> MNPSQTQKGKIQIQVSRGSIDLLVRTMYEDINNIKLKNERFQKKKRAEDERRRRERYAEIQQEAIASGKKNAALEMKWAELKELDECEELNREMQDQQQTFQQIIEGKENLRKEFEEELKRKDDEYVKMLKEQSNDIKDMISKMRSQFYKIRDANMQELEDIERHFEQERSNLLNEFKAKIQATFKKHLDLEEQYVKEHAKTEEEQTKNIEDLRIKGAKHYAELKITMETEIQDLEKCFEDMKALYQLITEKLDYSLKVLQEKFHENNSMCDELKRKENNFKNRLKQLTKDYKQYDKKFKLENKNLTQEYKRIIRQFKELQKKFKHFEKADLDKYSEIQKMNEAEVKELKDKIIKCNITIHIQQLGMQWIPPQSEEEILAQQKLQLEQGGKAEEEEEREFEFCISEIKIGEICNIILEEADFLIDDKLREELEGSAEPEQIFQRLDCIKKCLYIDSEDEMNLFFRELITKCRVKSAEEIEEEARKQLLLLGLIKEAEENENPEGEEVQQQEGAQQKKKEEGNKKDDPKGKEGAKDSKENANPQGQNKSNQDERKKKKDGQDDHAGQGQGQYDSNQGGMGENQEEGENAEGQENLEGEIEKEIDLENTQINLNEVVKFLQNWQANKDKRKEKLEKESSKKAVKQETEREKKERIAREGKKYWEKLTQVLPERTFRIWNVNFFKFSFEKQILLNQINKLRFWTDLCPNIMNFFWTDKNQSKKPVNCITKMKNQRIFQINTYKLIMNLLSALQDSLIQIKDKDDFIQTKISTNLFTFHNFQILLQIFIVNQSFLFIRLCQSYSKKIILLIKNINQKLFNLSNFKNQFSF;> MALLGKTLKGRSTRPGGIPQKRNIKWRQLAKNQEEFDQLKQLAKMKREGLKARIKDEQKVVTFNKKKLITYWRKIMRIAKTEQLKNEIDIYSQNNQRELDSKEAFIQMLDKNLDEAEDQFQIALRNHLIHIENLMQLQEARMRGLAEEFNRDVNILETEFDLEREEMVKTHKTQLKELEDMIETVKEEDKKKTEEAQNEFSQFKEETKNKNLEETNVMKIILETKQTKYYTELEQMNSKFQSDTSNKVKDHQFYHAHNKNRKQEIDRYLRTISSKKAKIDLMKLKILQHCKEFNARNSALKKEKENISRNYHELKLKMQKFREEESRRLKELSNNSRNAVLKLREYCALGEKILKTAELCRRLETEKEKVLPFYESSVDEDQIPEQLKNEFEHLKKEDAEEYAYLNNFYKRYNKVLLDKLAIEKQKENLQRDNQLLKSLLKQYLDGISLNDDVLKNENNPLLVVNHKFNLGKMPVEKIENKTVIEGVFEVRNTSHQLQGQRAPPFQ;> MSNYISNYVQSTIVTKTVQNKDKKTGKNSVDPRVINEQLILDAVKQFNQENNKITTENIILQQLRQLQLSFKNILKIQHLQGLERLEKLQLDNNIIEKIENIDHLVNLKWLDLSFNCIKKIEGLDKLKELTDLSLFNNYIEKIEGLHNNTKLNVFSIGNNRLKSYEEITLYFGYKPRGEEGTNDRPEFKRLQVLNVSGNPFTKDKENEYKNHIICAIPNLKYLDYVFIDEGDRQLIRQDEQISNSYNFTTTDYYQQMQAQEQKEEMDRQTLKKKKDARMDILDNLKDEYLKIEDLQRVKIIKPNQINEEIEKYCGKINDHVVEMQAAVIQKHQLILQEMSKTEVSYKEQEALHEKETLQILKEFEHEKKVEFRNWEKEAANGDAKKEESRLKTLLQKTTSLKNKLMDIEIQLVEELEAIFTDYDTKKKETAWKDIEEIIVLGQKKIEEENVKFYSNLNVIKNKEEANYNSTQQQQLEEENNEEDDEKASLLENKEQLAQMIGNIKETLIDSHTKIILSAQMELQKDLAEYAKQQKNKMYERNRKNISQIIAQIDAYQTEINEKLKQGDDESDHEN;> MSKAAKAKKNVPVVSKLEADARKAAEGVNDNESEEFKKAMRKEARALVEQFNEEKKLLAFYQQERQKINYNWIIAKKELEDKKSELINKEREIQDLQENHFMTLNVYKQKIKHLLFQNQDQQSELKKDVEVTLKQLEDQHRIKSRELKTDVRSLKVTKKEQEISQQDYLFALKSEHDKQMTLMRQDYERQVNDIKRKYDLKMQNLTKEMEEARAAMIKQLEDNKNQKIAEIIKEHTQKYNDIKNYYSEITATNLDYRKTLKNEIKELQTKDEEYKKTLQQTEKGYKELNEPLQALGIEIIQLKKQDEEQEAIIKEKEELKQKIDNQERLFRKLEYEYEVKLQQFQYLERERNALYAKFNQTVFEIHQKSGLENLILEKKVTNLREDLEIKDLQIHQVLTAANIDPNSVGSINKSLEEVESLKNELISELQAQLKQIRKAHSHMVKAYEGKLSEFVIPVEELGFDPLVPTNTD;> MPPKKAKGKKKKEEEPDDEYKSMTGADLTQTLEKLKERVNEMRTNRNYIQMDRDMVENFYHNTLKEISEVKTKISNKETEAEEKESKHRIDVKVFLQKVKHLEYEQEKSNLNIEDDGKKAKEKEDAYFEDITKNMKQLKTQLKSEYLEKEKANIQQVQEEKKDHQSLLKIQQKKFDELINNLIIKYEERLAKLKEDLELKLKVEIHELEERKNLHINELMNNHEKAFAELKKYYNDITAENLNLIKAHKEKIAQIYANIQLNTKNVADNQAKNEQLKEPLAKHREIRNKLKEDLKQFAKHKMSLQNLKSKAITLKDKITKLERDGKDLDEKYEKVVREKQELEKKFEDITQEVKKNADLNNNVLSNRLQILLKEYNNKEEELRTIIDNAGLDHNLHEQLKQRVQQSIEAKNTLIKNLKYSIHHATKAYNDAIRVYEAKLVEFGIPIEELGFQPLETITSSMPAGLVSS;> MLAKKLALARSQGKPDPFKKDEFPLLQHIAVEVVSQNYILYPDLKGVPENVRDTIISKITTDLDILTMAPNIDQESFWQRACKNRWEKSQKSINIEEHGRSWKVAYLERYMEEFLTNIQNADDPNKKQILQAELKAAASWIHTLNLQNINQNIDIDFICKYLPLLTSLTLTYGTKYSGMDYNKQSVGMKLSEAANLGEAIKNCYSLLSLNISANMIDDDLLRFIMAGVNMNISLIELNLSHNKIEDQGARRIAKFLMRNEILLYLNLGNNLIGYEGSRYLAQALKVNKNLQSLNLKLNNLGDKAGKKLFQDLMLNKTLLELDVSGNQFEFETALKLSDYVADSMCGLKVLNIANNDFNDSCYENLKTGFTKNYSLAKLDLRGNKFSKTQEEKEQELKDPFRMFNLSQTEKELTQIIIRHDLTAQKIQFFSESDLDKIKQLKELQGAKQEPEKVIQQDQNKE;> MGDKKGKKKGGGEEDESTLQLSRQYKKKCELNGINPSKLFKEKLDFAVEEDENIEKIHLWEELGPVGVRSIMDSLTEIPYLHTKSIRLWKVKAQDEGTRTICNYMEKSKTIEYLDLMDNQVGSLGCEFLGRVLHPQIEIPLLKLKLDHNEFGTEGLMQLAAGLCMNSVLEKLSLNYCAITAEGSKYIQQILSFVNTNLKKLKMKGNLLKNEGVHQLFRAFKVNKTLEKVDLSDNQFDTTLGDDQDPEANPNFFETNKDAIEHNKQIIENICEVLKAADTLLYYDFRFNNISKTDAKAIIDCLEANKNIYYMELSEHIPKDLIERKKGLMKKRKPKKKKKKKAKKK;> MDHNEGGYSHHQIEGQEGQQQQAPVGGGGEDIFQVLENITQVQNEKLKRCQEFKEQENIPRQYIENSPKEELVLEHVIQFKRQFQYQLYYEDKRDLFLYPKNECDVYKFICTTIRPTKLGFLELYDYQQCSKYLSEFVQYEELDPPNEFPLVIPSPTNVAVWQKGDCFDMSILLCSLLIGVGYDAYCVYGKAPREITTRNESLMECLFLEKGKYIEENDKKPKQTLEQNENALLKKPIAHSKWDQTQETKAREAEEEKRRIALTINDDEPDELLEDPYQGQRVHCWVLLRSGKRDVQQNIFIEPSTGRMYSPSTCPYECVDAVFNNLNFWINMKPECEVKNLNFEEMDSSLNWEYVMLDTLLFNKGNGNDEEGNENIDDPLNKQAQRDPEQEQLQDIAQLLDMPPPWPPKIYIDKEKFLMGTPLGEGTVYYNKVKVDNYAPYSQPDGLVQKITIFQDYKRLKVKEYRYFYKHRSDKLSIRRRYPFEFKTIEEYEPQKYENKTIPQALQQWRQVIQIDRHLRIIKYYHNRNHDGLIERVEQIGEKTMMFYQNRDDRVIYRSIRFDNKRAPSSQNNDKVFQDNHVGDVQITKMTQKFEKNPHYPANEQIQKMVIDLIKDKVIVYYHMNDGEITPIVKIYPRDSMHGFAKLNEPGGDNKIDDPLVQLENTKMVNLEKDCLNQLKQQEKIARDDEKTIREGEIRLEKTLYDKARDRFKESSKKNDDDLAKDAAASDYLYPYLEKRKLLGVSEINAQVAMEIKNEVMQKLKERLLSRAEIIQRRLEEQRQVLEQKEAQVAKRQEIDPKQEEEIRDINFKIDILEQRALRFESMALQKYEEMDNRLNKDARLAALHRK;>MYDPNTSQTEKQKQEEFLKLKIQEAFNLFVKDKKGIVDKREIPYIMRYLGQFPSEAQVRDAILPEIEEDEPSEFIKYSKFEPYMLKVLKEREYEPDDPEALLAAFKLLDQEGKGYIEIDMMKTFLEKQGIEFREQETKSFIEFATNKDPNATVIYYEDYISRLQAFTDKHIESVMKGYNNFQVKK[2x];> MNQIDAHKLTIILRDATERLTFLDTINRQDDLSSELAGYEISKLLKKQKNLENQYADLVQLRTSLTGIQNKKNLIETQTKIVDVAQNLKESTKKLCRLFKENPDLESDALKVKKDRIQFMAVIEQLIQMVQNNSLTKFQSMTTLELEDQDRLRKLIFREKELYQEIKKLQFDRNQENKEYDNEQKDTNLKIQNLKERLLYKKARAQLKNQYKEKEARAEEGTQQRMYEFEQKQLKEKINNLKQKTDTENMVHEQLRNFLIEKEDQIKQKSDEWAKKVETCREQLQEEIDRLTVEKEKKQEELRELRERDQKEQEEKDRRERQELEEADRKQQEELDQIRLDNAIKLIQIEYQEWKDAGGGKKKRKKGKKKKK;> MQNLSKMQSRLHPRPEGEGGGGGGRTKEKGKSLQETHKEMLKNIESTNIGKPTIVEAQRILKIIDNLSTNLTIFIYLDSELISKFLDVAKHSKLSKDLVSKLSQRCLDLLKSQAEIEAKFKPYASLLDQSNKEAEDVEEEKMIDAERLRMQLENNFKDLVRHLRNSPEDFEIIKSMKTNVNPDLNDLVHCIHCQKVIMLKKLSTASEEDENHKAQLRDLEEKIEELEKKKNKIQEDLTKLKEHRQKFSKEKKEELEKLKNEIAEVKAEKEKKASQLKNELDNRLKQLERDHLAKKDKLDKELQKLEDDFAKLKQDHANDETKLKTNKRQQQNSLADNIESYDALMKDQHQKKQEIEEELAKIIEEVDTLKQLFKEIDEEKQRERELEEEFRLKKEQWEIQERRKKEAARCILHFLMARKEKSKKKKKKKGKKKK;> MSNMMYNMKWQEAINDLMEQVTLEYLPLEQNEQQLGMKYKRDSSEWFHFWATLYIKYIDIYKKLEDCYDQLVHPQKRVLLKEMLENVIVRLCETKSQVVKYNTQYDATYKSDYPNLDELVMDLKLTPDCLDIPIPRYFREEDKKRLDERNQILDALLLEYTDTKEPQEEQYEDQNTLQADMDTAIRIIQRYERGRQGIERANLAKILKKEEEKKLERQKKLAEGTEIGEETEKDDAALVIKKYWRGYKSRKLVQDIREEELLFLGMKKVVEDPTLPESQYKQAQNKRQKMKYIQEEHEQEFNDEIENLKRLVKGNEGPDILDKMRAERREWIMRELEKNEFKEAPQDPSEFYNQQVMDPEQQAAEAAKAAEEAKKKGAAKKDDKKKKGKPSELDEFLENNKPTGPSPIVLKLQEQIEKHSGEWSKRDETNNFEQKHETELAKMLIKPVVEEQIKQQVDEMIAEELDIVRLRYDIKKKKQKKPPRPRNKGKNKKKFPGDSSNKGRDPKDILAGLVEKRVAKKLIPASLMDLKGEQNVLGKIQEIQADENLKKTEALTDAKLKKAQLEEPSTKMPDPSIAQIRQIIAEYIAFPLGSKYAKEKLDKMNYFFFMGPRGSGKTLAVRALAHECNAIVLDISPSNIDGQYTDKKQIDGMINSAFKVAKEFQPAIIYCEDFEYIFGQAKKKKSQVNPLFAKMKKPLMDFKKGKFFEPEDRVVFIGSTNRPWDCSQKEIKSFFDKKIYFPFPNYGTRMLLFKTFLEQKKVPLPDNFPINTIAHITEGWSAGSFKMAIDRVFTERRLQKINEEQIKLSEFIGPLSNVPFTSKEEFKEFKKFNQVVTGLQANYEAKKAPADDQKGDKNKKKK;> MATTTNILHDVVRDQSMVNYVSNRDRPLYFKRPLVPQMTDIPLHISRPPVDQQVDYQTMQMQQNATIVEAPTKDAFVQTDYRESETQTDPYTPKCFVRDGDHPEVMELKDYKYGKGLPASIEELEQIELNREKVWFENSLPPISDEASFNLRRKLMEEQELREWSKKENEIKKFQNEKLYLLQQALIEREKEVEDKSQERIEEIRQQKTEHKNRQIAKIQRKKIKIDRKMTKSRKMQGKETLKRDIIEDYANFASRVYAGITHEGLSLDKIANKYEVQPLALGNYEMLQALHEGIRPREFETRVNLKKEIKEIEKNYTRLENYHRGELKKAQDEINGVHEQSKAQQKQEGNNFSYRNFENKIRPATPTWKYDTDFNISPSLITEIQEYRGPNGVQLMQAADKREEAVLLLQRLLRGRTTQNIMYEGKKKRTALIEELLTVAQIENLEEDKAEEVLMQQHEEKVKNAVLESIQGEVIAETMDELSKELLRIKQERKIQQMVEIAEKDRRIREIEEAGKRQAEEILRDREDVLHNQLIRVHQGTVDTYLDWLMSNALEQSSARQATIMTNLRKAKFNLPLEDFERKYNNNQTLIKDLVHSFLIPNVQRSKLKKQIQLEEKRFSEAAKRSLQQTITRASNKHANVQN;>MDQGEFIQDDNDQDYDQQEGDDENNDYMEDPQQDNNYNQNGDNLDDQGQDDDGGQNNLQQPSVPPEDDEDDDDDFPEYANEQNKRLNEIIKKKRKLIKDISAKIEEKSDRTKVLQEHLKNVEQELLHTQALIDAKNKEIETEDHMKQIAERQSGRIQSELKILEKRSIEQQEKLNDVQNQIFRGNEKMDQYKLEMNWNQEELEQWALAARQKEEDNLTLEKYKRADEVKIKELNLAIEKLTAEVGRKQNELEKEITETQAAQIELDKTAEEFKRQHEERHKLFLQWQEVTEIISKRDLAIREEGENFARIKIEIKSNKDALEERKRILKEAKEENKRIQMANELMERQNIQQISDNKHIEEQLAEKKADVEILKNQVSAFASDLSSKKNRIAILSQELLAKKQRLNAAQKKYQAHQVKLKNEEIMAKQYENDRSYAEEKYRKNEKEKKELEKEIRTQKENLFKHTQELFKHREREANLYGEIQGNMAACRNLQSHITKLNQEFQRQQELLYNAEYQIQLMERRVARAKGERTLEEKKDLENEIMNAERELGGVTGQNKELIESLKNLDDEIRTVKKKLAYVEEENTKYSSLIEELILENDMTYQDLNKIIKQKEEVLVQHDTMKLEIKKINESLNGATEKVFNLENQIYQLEMSMQEREKEIEVHKDVLMTEHKAAEEERHKIAVELAERKNKVKNLKIKYESLVQKNKASNGEVESVHEHSQAYYVIKAAQEREELQRKGDELNAKILKNEKELKALDNTLNHLKNRNSNYRDKFLNKGVTTQHREEAEGLEEQCRAASQNLFKKRDELQKLQKEQEEDTRRYTEIKNKLERLYEQHQSLDQEISKYQKDIDQQGDKLQRAQNSLQRNYQLAVNKNQNFINPKNPHMIQVKLDNQNNLYKTLLQGLYSLQQDIPELSSVVDEILKEQRIQNNKAPSSIDINSKRSSQSGRSQRSQRSNISNQ[2x];>MSNQQGPEDNNLEDDMAYLPADHPLLAKLQIDLTKQLTDEHERVDQKLIEIDANLKKLEKTKEDIGVRLYSVQQQLAENQMNFEQAHENYNWVQKLRIEAEQKLKTESEVYDAKKKELEELRKKYLKAQDELSKLTRTLYQINEFNQQMKGQIINTKTNTYRAEENVVNLEAQKKKQDLLIDTMNEEIKRQTEQKTILTAQLISQKEETEQAKQILKEAHLEMQKIIASKKNLLERWQKSLMTMQRMDNALQAIKEALKGQQELNLQIGTELNGVNAEIRKETEIQESLEGKNKKFDYEKDYLQKKYNELQEEKSKLEAQINLLTQSLRQTETEAGRAEIDKRNIEDQMNLIETNIMKLHTETKKLWEDLVHQKSEHTTIEKTATNLNKQANQISIEIEDKSVELENLLNEIARVKIDQLNTLSQIEVLENKRREVIKEREEKEITVATYEVQIRQGHDLNEKKQHEVGRLNREHDKLSSVQSDMSRGPLEAKRNNLIRKTQELGKENDLMQREWIKKQTLLVTQNNRLNKIEEDVSQLKTKQTILEQKKLRLNNNYRIYEKDIREIQNALKNLRNEMNKLNDAIYRNKEKQQKLDNENFNIKSEFVEKLKELEKESVKLEVEIDRLKEEKADLLAEIVESERQILLWERKIQLEKEMQDALDPTVGQTEIQELKREIHRMELRLDDLRKKQEAIIAEMERAVYKRETIQLKYMNKDKTFSNSNSMSQKSSSISAASDNSAQITKKIAQLKTTLNQTTRNAEQMEKAIKNKKIELDDLNAQIEGNNDNLQKLESDCYNKNIELTKHKLERSTNILSISCMQNKAKKLEDLVAGKARLSVPEATLMTKYEELRDKNQEIKEALQKLCDDAPQYVEVLNYLIDLNVGDDDEDQEQ[2x];> MASEDGEMPSQFEGIDPEQLTESQMQQYMMEMQRQGLLDSNMEGGQYEEGYEEGQEGEGYGEEYGDQDYDGNQNEYDSQQDSQQQGHDQVNEMHQDRYDRRVNSEISGNYEADDETLRKIRRDLLDNINLERRHRDLQPVYIDLTTNNISQYYSEYLVNNEHNQDFYENAKVRYNNLGECELCHITAKFEPDADITKEYIYDYFMEIGYLFLESEEEKRIILNPANNHIGIGVFFDEIQIVVVLILSEKVLCIQKISQPEQNKIEIRGKMLDENFGIYAIRIMNVDDQKKDIKGVGPEFIEYTRSTQEWMASFELELYNQDRMAIEYYTRVSPDSIPYKKKQSKNEKLTYKHLQLRLRTPFQIYPDPKYAAEDEKERIRKEQEILAHEEQERKEREENDAKRLKQSRKDYGDGQYDDDEHGQDDFNSQSDISDKDKHHDSMHAEQEQNQQAAQQQQDTISNKEIRQELEMAITEAQRQHDEFMLQNHKLQEEIKLLKNKNDGFVDRSNETAMNEHKYLNTLAHVHQIRLDLKQTQTRYNQMSQELQKKLEQKQKKCNEIKYAFLELKREVAKKAANSRTDKPIPEQQINEWEKAELQKSKELQELRLQILRLRNAYVKNQKILKKKEELAEGLHLIDFEQLKIENQTLNEKIEERNEELHKLKKKNTTTIQILTHTREKLGFVQGENGELNSQNVRKDQELDDMRKQLTQQKKTKDKLRSVNLTLKQQTGIVNSEELGQDYRDLRTRVSKLEEEKKRLEQKLRSMHEAIKTANQISTQNMQSQNNSLKKPYQPY;>MDNTGKLEKQLVTLNDGLPKKPAKEIIEELKHHLYQDFQKFFSEEKKQQYQNNFALFDRDNDKYINLSELKELLTSVNITFPDDELEELYNEFCLTSPEADGINEDAVFIIVSKKIRDNDKDEQLTQAFKLVEKAVNDELAKTPNETKEQEGYIRVEQFKELLMTLGNRWSEEQANEFLKDINPKSDERINYLDVVKKLMKR[2x];>[2x]MSKKSGKGKGKNDGDELGAEKEQVLRTKVESLIQRLGHEQERADRAKAAENELRARLFDLDKDFKNEKDRLFSITSDMTRQYKQMQDELLNQVNDLNKTVIEKDEEIKKKDQQIQDMTKDYEYKLKKKDDEIQDLKRKIEEMSAEFAKMLKDTLDKMQERIEMVQWDSDTDPQMMKRLKDMTGLSNN;> MNQDKHPEITDEEQELITVEELSQKLELLYKDMEQIRRENLLFEAYLARNRKEIAKEDEVSEDKKGKGKKKDKNVDKKSLLLTNEEKFEIAQQEQDALKKQIDDGRIKSDQILETLRAILEETDMAITEIRKDAFDFQREILVGGENSRTGKIEAEKIIKFFEEKERQKDALIAKYSSKRTNLERQILKTNNQIQKKEEMGDDLKFIDFYQLQIENKKYVKEIDDKNKKLLALKISTNRISQTLKDEKQNLKQELDKGKEYASQMSERKKKISKIDAQIKSVKKVTSKLEKDRKIYDKQKEIFVQDNQDDVPQIMKYVQYKSKEQQLLYAIQNLERKIEIAELAYKKANRILQSSQQFQQK;> MAGLAQHIQLKYIFGMNNEIRNSLQFHDEDRIIYPAGYNVVLHDLNDKSQHYYQGTNEYRGISCLALSPLKRYLALGVKGQRDPAIIIFDTFTQKRRKNLGLNLGNLDRYNIKQWVSIAFPSQNQETKYIFSLSGAGGDVVLCWWWHEKGKCLGSIDLGAQNDIYEISFNHSDANSICVTGNNFFGIYAKIEGTYVREDNQQKQKPSVQNGENSSAAQLPQPTLNIQVSAGNNNQNPQPEIKLENGNLISNLPADIVEKNFVAHLWMQCESYLVVFVESGEIILCDSRGNFLQIMEQSPRYFIVSRSGMIKIVAAVAYSKGFYVACSESIVLQYHYTQDNDKNPFTCVNQFKLKQFVELKEIEIKSICMNKAEDKLLIGLDNNQIYEIKIKPYHPETVNNDSSEDREVTLINHLNHTGPINSMDICKRKPIIATCSTDKTIKIWDYEKKQIKISWAFNEEAFCLSLHPQGFCVAVGFLDKLRLMNLCIHNSQNTTKNKAYKEISPFKGCKEIKFSNGGQYFAAVNSTSSNHVIQVFKFFTGENPSQLVFKGHTGRVKCIAWSSDDSFLLSCGLDGMILAWKLDQDFQHQQTIVPRIVDIHNKGVNFSGLTLTVDNKTIVAVGNDRHIHQAVINEQQPVDKTDKKLLDINLSCLAFPSSNKLLFAGIQDDARSSGAIRCFIYPLTHGKFTDYQAHDERGVEKMKITNDDRYIITAGKDGCIMVFEIKDKDARGMKLKDGYAKYSEEELITRSDLDDLKSTRDGLIVQINEFSNQNAMIGLNSRDDRIRQLETQIENNSQKRKQMFEQLLKSKTMEEQKLIQEINEIKEQFEQEIQVMDTKYQKEVMSLVEEYENQKRLHEIENNKNNKKKTKLLQEHSQKLQIIDDQYQKLLEEQITQKERVEKQINHLQKEQQEVLMQISEEKETEIKNLNQKNSKDEQAITDQGLKAKSDISITKKKIMQQQQEAQDLKEQKQEYERQKEKLKIQNQELRDKIDGQKKIILERDRTIGEKEKIIYNLKKKAQDLEKFKFVLDHKIKELKRDIVPREDEITKMKQETNNMDQYLKELNAYNNYLGTVVDELYTTQETMKEDIKQQRQQISVQQVKISRFKDDVYSLAQHILDYDKLVDETERLFMKHVNDKEVKRQSVEGDIMMEYRSQKKNLEKLVNMFKKSLQKDNQIHKDDKIRIMKDNVDLIREINTLRKSIKDITKGQQSNIPDQKGQTQHMPLQTPQLSRKSISQPVLPPISKSAMFEGVTQQNEIQKSHTQINPELVEEKQKVLNSLQTDILELQKVYEALNYEKHNLTQA;> MSSDVKDSSHLEKQNSQEYSNSKQNGEIDIMEMLPQKKMYIIEKQFDQSGKGLKIDEFVRVMLTHLDFDKSDVQKEDQITLALIDLFKEIDVNGDGTMEWEEFSDHIISLGLLRNDRSFKNVIKNYFPSEHIKDNQKHETPIEKIVYFDKLKYLVVLEKDSTRFKVYNANTAELYYEVNAHKCAVLDAEYIPDQNLIATSSNDLTINFWDSSFFIPKQIVSVPEIQLCMRYAKWSTQSQPTYLYTGGSDSIIHIYDTKTLKEKGTIGGWNPFFKRDSQQYGHASPIGDILPINIQTTLVTAGLDANICLWDAATHLPKKELRGHEKGVYSLDWSDFSPMNQCLLSAGLDHEAFVWNTYVKEKIFLLRGHNHPLIGVKCLPGTPQVITADINGMVKVWDVRNFLCMQTINVPTDELNSFVVTSNQKKRIIFGARRLYYYEYDEPKDQMLTDEKMCLRVLYNSVLLCLITLHPDCIKVWDIRTGKLQSVYRELSTAELTVCVLDTRKRKLFVGDADGNIFTVNIKNGAKMKKFEKHNNRMITDLTHWTSKKPATIEIGGDDDDEDGTGDSRRVVSCSREETVFIHDEDSSDPSRSCRYKMKQHKSSVNSLSLKQDSELFASASDDGNIVITNLNSYRQETLPSTQYPFEKKKVIFLDPYNALVTSDSEGYVHFYCVNNGKARTRYLLTKKYETTSVVNNKVDKFPVTHLAFNSDNNMLLLSDELGNVTIWDLTIFLKKLDEIKDDNIQQQKTKQAQTPLKQTPNRASNGFFPTELDELKQINEKQISLSQMDNLEKYFQDKDIAFVHQLKGAHNDGITWIEVLKEYNMFATSSFDCCCHLWSFNDYKKMGSLILGHDIMNNNWQLRVDEEKRKVDAQYYMEKLKKKLNKDDQSDDEEKNSQKQDESMMSDKNFDQKNQKKPKKTEKGEKGEKAPEKPLPEKKKVLTAQEKMEQNKKLKNELKLEFDPALLNLNKNKKQVLSEKEQIEKASELLEKVKKFNDVIANKNKDRRNPLEIDYDDFLRAYQMDEQVDIYLDQNEEEEEDNNILYDLDDPKNQSIPAGAYTSKGAFKSKNIGRKNKI;> MFKNTFQSGFLSILYSIGSKPLQIWDKSIRNGHIKRITDQDILSSVLEIMGTNVSTNYITAPADPKETLGIKLPFLVMIIKNLKKYYTFEVQVLDDKNVRRRFRASNYQSTTRVKPFICTMPMRLDEGWNQIQFNLSDFTRRAYATNYIETLRVQIHANCRIRRIYFSDRLYSEEELPPEFKLFLPIQGQNKTNV;> MAQQIVQSLQDEGTQSLKLDFSMKYVLGYRSDFKNNIFQYTMNDQNRIIYPAGNTIVISNNENKQQFINCIPGTKGITCMTLSPSKRLLAWSEDCDSGIIVVFDLIKLDKLEKAKNQNYQEPSDKDKLDKQAEKDRRDRFEKEKREKIDKLQKEVKRIITTLDCKSRHYVALDFNKINEKRIVALSCAPDWQLIYFQLDKQKTVIINQVPLKVGDNMRYTHCFFHPKEEDFIVAIGTGAIKPYKLGADGQFKQKDPPFVKKESKDQA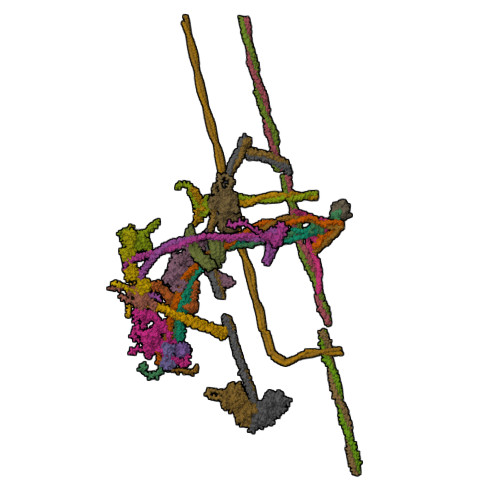HSPNYLSYCILQDGYMVIGTDMGEILLFQPSCEFKTILASSPKNEQFAIQCIQPYSKGFLVGGKECTILFYEKDVDLKNPYKLCSKKIQFRDMKAMITSLLLTPNEEKLIVGVDSGQLLQVPFTSDSMQLNEENSKCEPLFMPFHSDKITGLDVCIRKSLVATCSVDKTVRIWNYSDNQLENSKEFEEEAYAVAFHPSGFHIIVAFTEKIRLMNIFENDLISFKELSVKNCREIQFSNGGHFFAITNVSMVQVFQFYTGENPSNLVFRGSGKVRTIFWEEDDQGFYTGSTDGLVIYWRVDDNGPQKTQIAQFNNLIITSITGLYNPDTTTQGLERILFVSGVSSSQENEGEKCVYKLVISCRQDKEGREITDNTLKKIYYVSQPEQKIFTGTNVSQIAISHSKKLFFFATEDRPGAIRITKYPFTNEIMEIQSHFGPITRMRISFKDNYIFTAGEDGALIIYENKEKEYQVKIENESVEAAAEEFLIPRDQYNDQKREIEKLKRQLNEERMKQEQQIKEKMKDRDDKINQLENQQKDSDNRDLNKYQLLEREKNEMIESYEEKKRMMKLQHENNKRTIENEYKKKIALEMSRNEELAREKEKEEKRFQSEIQQYQEEHLRQMEEKRRHYEEQLAIEKQLYNDLHLKREELAYKFDQKRNKLEMEAEELIDQLKEENESKMQVLFKNLEKAEIKKMDRRNDYDTEAQKLEEQKSKLKGTMEDITSIQETNKMLQKEKESHAKEIDEREKTIRDKGRRIYELKKKTQELEKFKFVLDYKIKELKRDIGPKEEEIAKMKEQIANMNSEILHFKRTNANLKLIVTDLRLRQEGMKKEIEDQSKVIQQNNQYIKAFEQDMSDCHQHIADYKKLKQKVLNLYNQYVQGDDSKKKRLENNDQQKEIMKERAHLETSVNNLKIKHDKNQSVHKSDTTIIMKHNTFLIFEINHLKREKKKILEDKAKMLMQATQKKKQDGTSRVDIDSLEKEIQKNEDEKRKLKEDIEKLRQYNDQIKNQLRQQIQNQQDDDEDN> ALFGTKDTTTAHSDYEIILEGGSSSWGQVKGRAKVNVPAAIPLLPTDCNIRIDAKPLDA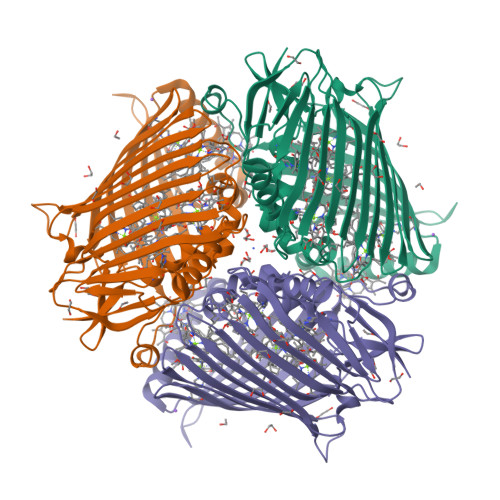QKGVVRFTTKIESVVDSVKNTLNVEVDIANETKDRRIAVGEGSLSVGDFSHSFSFEGSVVNMYYYRSDAVRRNIPNPIYMQGRQFHDILMKVPLDNNDLVDTWEGFQQSISGGGANFGDWIREFWFIGPAFAAINEGGQRISPIVVNSSNVEGGEKGPVGVTRWKFSHAGSGVVDSISRWTELFPVEQLNKPASIEGGFRSDSQGIEVKVDGNLPGVSRDAGGGLRRILNHPLIPLVHHGMVGKFNDFTVDTQLKIVLPKGYKIRYAAPQFRSQNLEEYRWSGGAYARWVEHVCKGGTGQFEVLYAQ> MKLNYFQGALYPWRFCVIVGLLLAMVGAIVWRIVDLHVIDHDFLKGQGDARSVRHIAIPAHRGLITDRNGEPLAVSTPVTTLWANPKELMTAKERWPQLAAALGQDTKLFADRIEQNAEREFIYLVRGLTPEQGEGVIALKVPGVYSIEEFRRFYPAGEVVAHAVGFTDVDDRGREGIELAFDEWLAGVPGKRQVLKDRRGRVIKDVQVTKNAKPGKTLALSIDLRLQYLAHRELRNALLENGAKAGSLVIMDVKTGEILAMTNQPTYNPNNRRNLQPAAMRNRAMIDVFEPGSTVKPFSMSAALASGRWKPSDIVDVYPGTLQIGRYTIRDVSRNSRQLDLTGILIKSSNVGISKIAFDIGAESIYSVMQ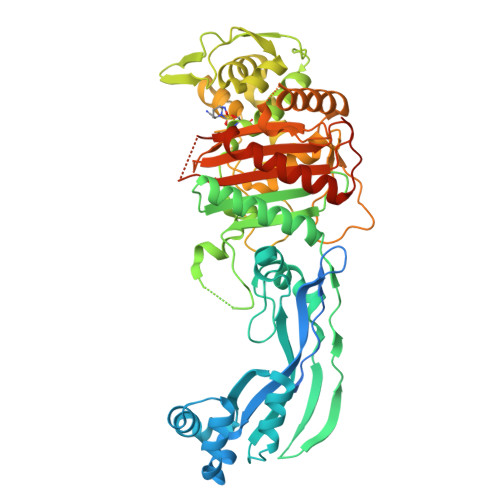QVGLGQDTGLGFPGERVGNLPNHRKWPKAETATLAYGYGLSVTAIQLAHAYAALANDGKSVPLSMTRVDRVPDGVQVISPEVASTVQGMLQQVVEAQGGVFRAQVPGYHAAGKSGTARKVSVGTKGYRENAYRSLFAGFAPATDPRIAMVVVIDEPSKAGYFGGLVSAPVFSKVMAGALRLMNVPPDNLPTATEQQQVNAAPAKGGRG4-[2-(hydroxymethyl)naphthalen-1-yl]-N-[2-(morpholin-4-yl)ethyl]benzamide | C24 H26 N2 O3 | 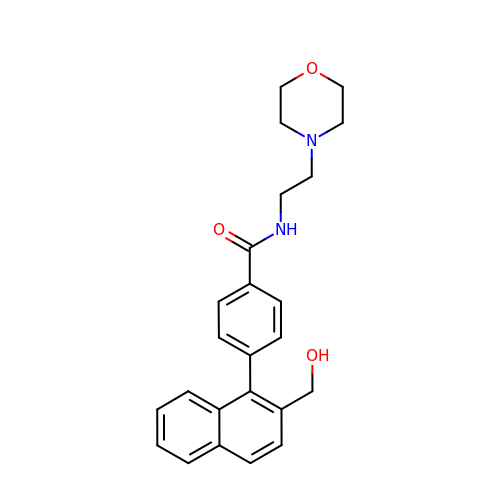QFHPEAOPPKNNMS-UHFFFAOYSA-N> KPEPTDEEWELIKTVTEAHVATNAQGSHWKQKRKFLPEDIGQAPIVNAPEGGKDDLEAFSHFTKIITPAITRVVDFAKKLPMFCELPCEDQIILLKGCCMEIMSLRAAVRYDPESETLTLNGEMAVTRGQLKNGGLGVVSDAIFDLGMSLSSFNLDDTEVALLQAVLLMSSDRPGLACVERIEKY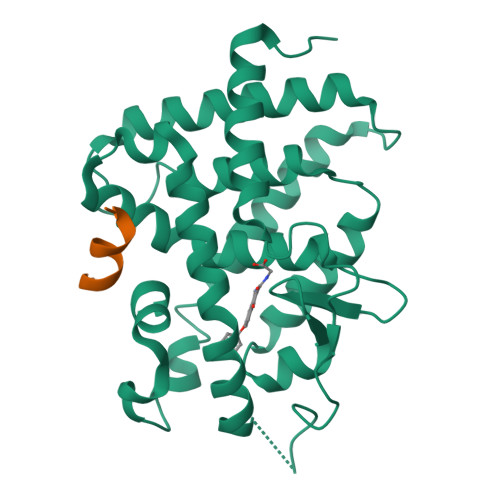QDSFLLAFEHYINYRKHHVTHFWPKLLMKVTDLRMIGACHASRFLHMKVECPTELFPPLFLEVFE;> ENALLRYLLDK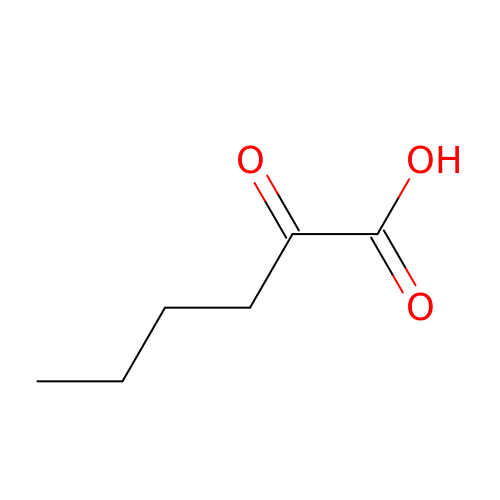2-Ketohexanoic acid | C6 H10 O3 | XNIHZNNZJHYHLC-UHFFFAOYSA-N> QAIKESYAFAVLGEPRYAFNFNHFDYVNPAAPKGGQITLSALGTFDNFNRYALRGNPGARTEQLYDTLFTTSDDEPGSYYPLIAESARYADDYSWVEVAINPRARFHDGSPITARDVEFTFQKFMTEGVPQFRLVYKGTTVKAIAPLTVRIELAKPGKEDMLSLFSLPVFPEKYWKDHKLSDPLATPPLASGPYRVTSWKMGQNIVYSRVKDYWAANLPVNRGRWNFDTIRYDYYLDDNVAFEAFKAGAFD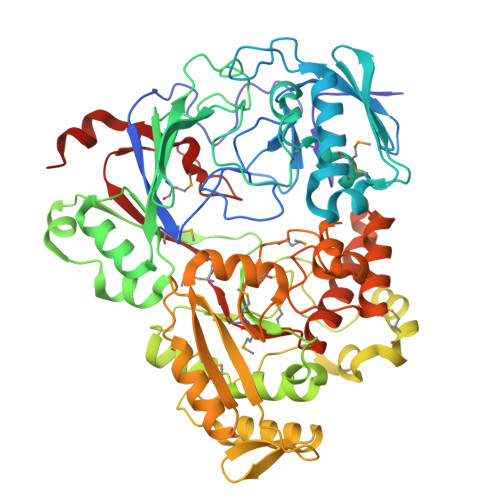LRMENDAKNWATRYTGKNFDKKYIIKDEQKNESAQDTRWLAFNIQRPVFSDRRVREAITLAFDFEWMNKALFYNAWSRTNSYFQNTEYAARNYPDAAELVLLAPMKKDLPSEVFTQIYQPPVSKGDGYDRDNLLKADKLLNEAGWVLKGQQRVNATEAQPLSFELLLPASSNSQWVLPFQHSLQRLGINMDIRKVDNSQITNRMRSRDYDMMPRVWRAMPWPSSDLQISWSSEYINSTYNAPGVQSPVIDSLINQIIAAQGNKEKLLPLGRALDRVLTWNYYMLPMWYMAEDRLAWWDKFSQPAVRPIYSLGIDTWWYDVNKAAKLPSASKQGE ethyl (2~{Z})-2-hydroxyimino-3-oxidanylidene-pentanoate 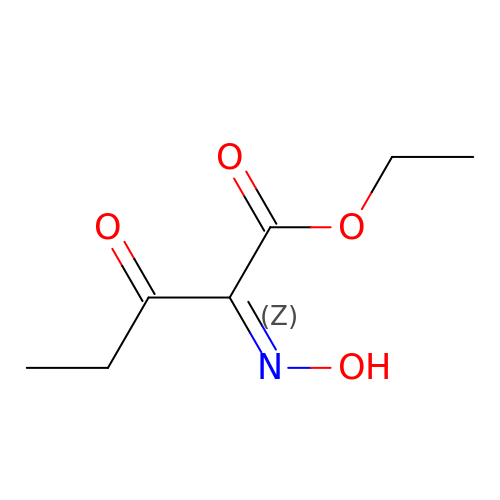| C7 H11 N O4 | FOGXVRUMMPWXRL-VURMDHGXSA-N2-(3,4-DIHYDROXYPHENYL)ACETIC ACID | C8 H8 O4 | 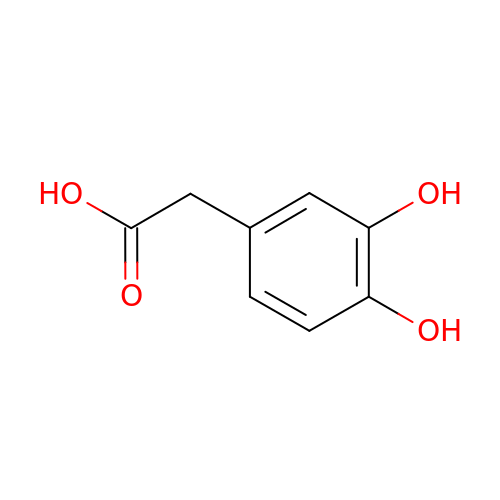CFFZDZCDUFSOFZ-UHFFFAOYSA-N> MTELCPVYAPFFGAIGCASAIIFTSLGAAYGTAKSGVGICATCVLRPDLLFKNIVPVIMAGIIAIYGLVVSVLVCYSLGQKQALYTGFIQLGAGL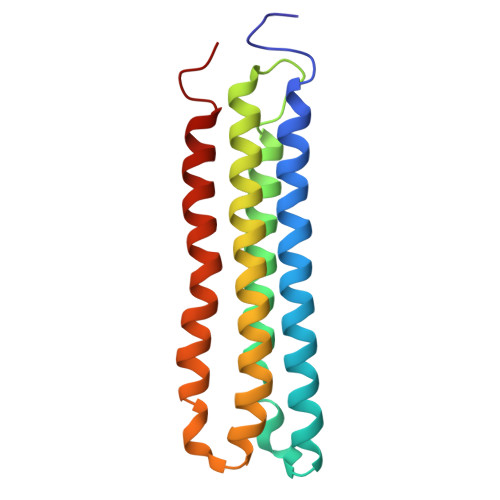SVGLSGLAAGFAIGIVGDAGVRGSSQQPRLFVGMILILIFAEVLGLYGLIVALLLNSRATQDVV>GSHMIRLAAIDVDGNLTDRDRLISTKAIESIRSAEKKGLTVSLLSGNVIPVVYALKIFLGINGPVFGENGGIMFDNDGSIKKFFSNEGTNKFLEEMSKRTSMRSILTNRWREASTGFDIDPEDVDYVRKEAESRGFVIFYSGYSWHLMNRGEDKA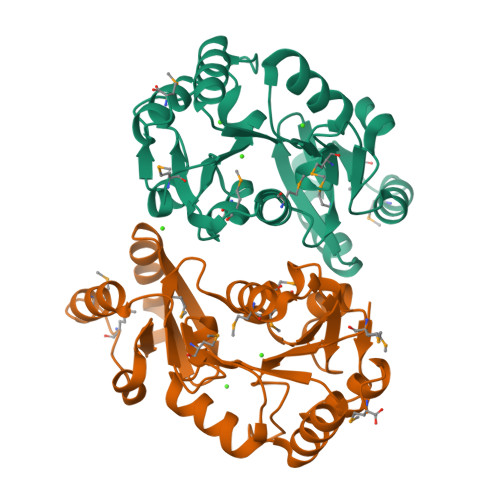FAVNKLKEMYSLEYDEILVIGDSNNDMPMFQLPVRKACPANATDNIKAVSDFVSDYSYGEEIGQIFKHFELM[2x]>[12x]GAMAQLAAPLKVGAIYTIGPYLFPHLIPQLHRVAPQMPLYIEENFTHILRDKLRTGELDAIIIALPFQEADVLTKPLFDEPFYVLMPADHPWTAKASIDSELLNDKS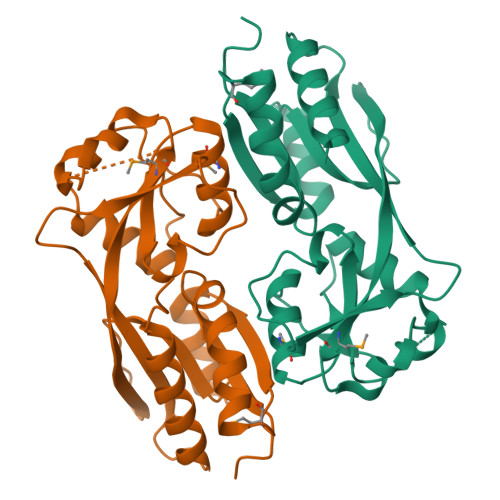LLLLGEGHCFRDQVLEACPTVRKGDENKHTTVESSSLETIRHMVASGLGVSVLPFSAVDSHHYAPGVIEVRPFSAPVPFRTVAIAWRASFPRPRAIEVLADSIRLCSVARPQTQEQPQIA>MSQQPGVLPENMKRYMGRDAQRMNILAGRIIAETVRSTLGPKGMDKMLVDDLGDVVVTNDGVTILREMSVEHPAAKMLIEVAKTQEKEVGDGTTTAVVVAGELLRKAEELLDQNVHPTIVVKGYQAAAQKAQELLKTIACEVGAQDKEILTKIAMTSITGKGAEKAKEKLAEIIVEAVSAVVDDEGKVDKDLIKIEKKSGASIDDTELIKGVLVDKERVSAQMPKKVTDAKIALLNCAIEIKETETDAEIRITDPAKLMEFIEQEEKMLKDMVAEIKASGANVLFCQKGIDDLAQHYLAKEGIVAARRVKKSDMEKLAKATGANVIAAIAALSAQDLGDAGLVEERKISGDSMIFVEECKHPKAVTMLIRGTTEHVIEEVARAVDDAVGVVGCTIEDGRIVSGGGSTEVELSMKLREYAEGISGREQLAVRAFADALEVIPRTLAENAGLDAIEILVKVRAAHASNGNKCAGLNVFTGAVEDMCENGVVEPLRVKTQAIQSAAESTEMLLRIDDVIAAEKLRGAPDMGDMGGMPGMGGMPGM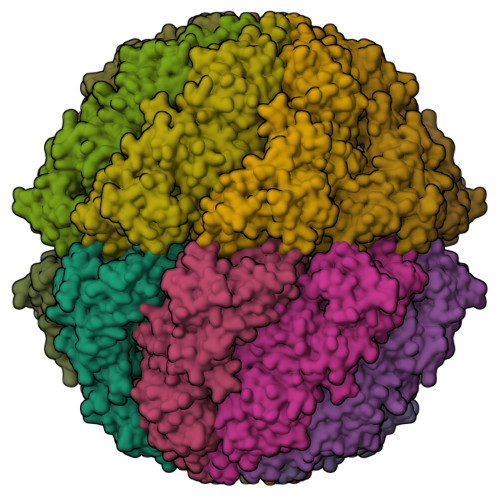M[4x]> SMGFWEASSRGGGAFSGGEDASEGGAEEGAGGAGGSAGAGEGPVITALTPMTIPDVFPHLPLIAITRNPVFPRFIKIIEVKNKKLVELLRRKVRLAQPYVGVFLKRDDSNESDVVESLDEIYHTGTFAQIHEMQDLGDKLRMIVMGHRRVHISRQLEVEPEEPEAENKHKPRRKSKRGKKEAEDELSARHPAELAMEPTPELPAEVLMVEVENVVHEDFQVTEEVKALTAEIVKTIRDIIALNPLYRESVLQMMQAGQRVVDNPIYLSDMGAALTGAESHELQDVLEETNIPKRLYKALSLLKKEFELSKLQQRLGREVEEKIKQTHRKYLLQEQLKIIKKELGLEKDDKDAIEEKFRERLKELVVPKHVMDVVDEELSKLGLLDNHSSEFNVTRNYLDWLTSIPWGKYSNENLDLARAQAVLEEDHYGMEDVKKRILEFIAVSQLRGSTQGKILCFYGPPGVGKTSIARSIARALNREYFRFSVGGMTDVAEIKGHRRTYVGAMPGKIIQCLKKTKTENPLILIDEVDKIGRGYQGDPSSALLELLDPEQNANFLDHYLDVPVDLSKVLFICTANVTDTIPEPLRDRMEMINVSGYVAQEKLAIAERYLVPQARALCGLDESKAKLSSDVLTLLIKQYCRESGVRNLQKQVEKVLRKSAYKIVSGEAESVEVTPENLQDFVGKPVFTVERMYDVTPPGVVMGLAWTAMGGSTLFVETS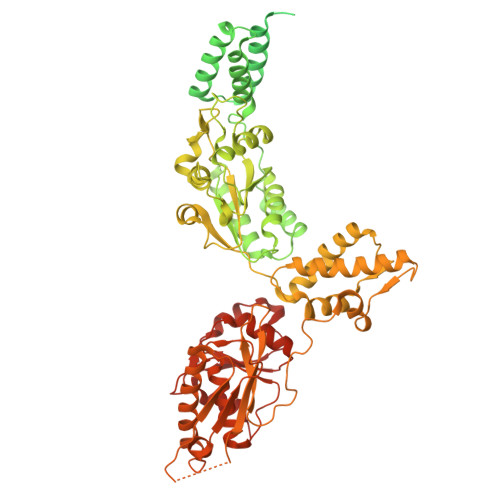LRRPQDKDAKGDKDGSLEVTGQLGEVMKESARIAYTFARAFLMQHAPANDYLVTSHIHLHVPEGATPKDGPSAGCTIVTALLSLAMGRPVRQNLAMTGEVSLTGKILPVGGIKEATIAAKRAGVTCIVLPAENKKDFYDLAAFITEGLEVHFVEHYREIFDIAFPDEQAEALAVER>[4x]GSHMKNPYSNQIEREELILKYLPLVKAI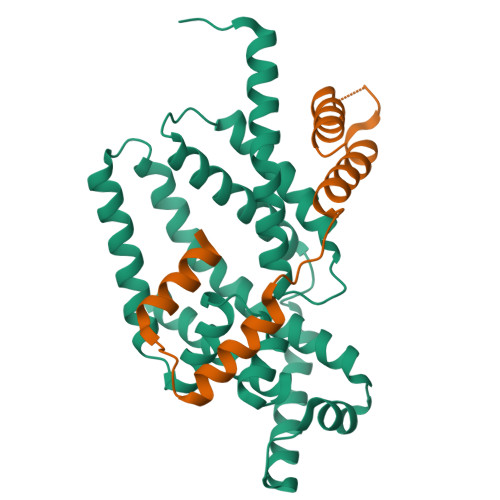ATNIKKHLPEDVDIRDLISYGVIGLIKAVDNLSTENPKRAEAYIKLRIKGAIYDYLRSLDFGSRQVREKERRIKEVVEKLKEKLGREPTDEEVAKELGISTEELFKTLDKINFSYILSLEEVFRDFARDYSELIPSSTNVEEEVIKRELTEKVKEAVSKLPEREKLVIQLIFYEELPAKEVAKILETSVSRVSQLKAKALERLREMLSNPL;>[4x]MVNRIELSRLIGLLLETEKRKNTEQKESGTNKIEDKVTLSKIAQELSKNDVEEKDLEKKVKELKEKIEKGEYEVSDEKVVKGLIEFFT>[6x]MNHKVHHHHHHIEGRHMRILFFSSQAYDSESFQASNHRHGFELHFQQAHLQADTAVLAQGFEVVCAFVNDDLSRPVLERLAAGGTRLVALRSAGYNHVDLAAAEALGLPVVHVPAYSPHAVAEHAVGLILTLNRRLHRAYNRTREGDFSLHGLTGFDLHGKRVGVIGTGQIGETFARIMAGFGCELLAYDPYPNPRIQALGGRYLALD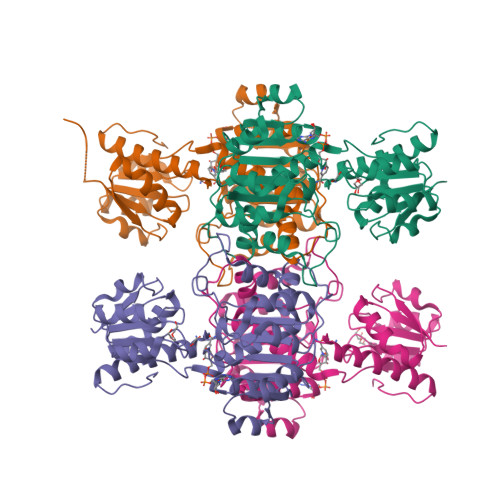ALLAESDIVSLHCPLTADTRHLIDAQRLATMKPGAMLINTGRGALVNAAALIEALKSGQLGYLGLDVYEEEADIFFEDRSDQPLQDDVLARLLSFPNVVVTAHQAFLTREALAAIADTTLDNIAAWQDGTPRNRVRA>GAMGSELNDINKIELKNLSGEIIKENGKEAIKYTSSDTASHKGWKATLSGTFIEDPHSDKKTALLNLEGFIPSDKQIFGSKYYGKMKWPETYRINVKSADVNNNIKIANSIPKNTIDKKDVSNSIGYSIGGNISVEGKTAGAGINASYNVQNTISYEQPDFRTIQRKDDANLASWDIKFVETKDGYNID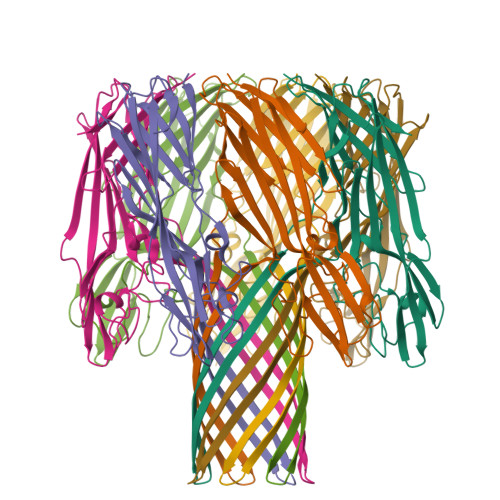SYHAIYGNQLFMKSRLYNNGDKNFTDDRDLSTLISGGFSPNMALALTAPKNAKESVIIVEYQRFDNDYILNWETTQWRGTNKLSSTSEYNEFMFKINWQDHKIEYYL[14x]(1~{R},2~{S})-2-[[(5-bromanyl-1~{H}-indazol-4-yl)amino]methyl]cyclohexan-1-ol | C14 H18 Br 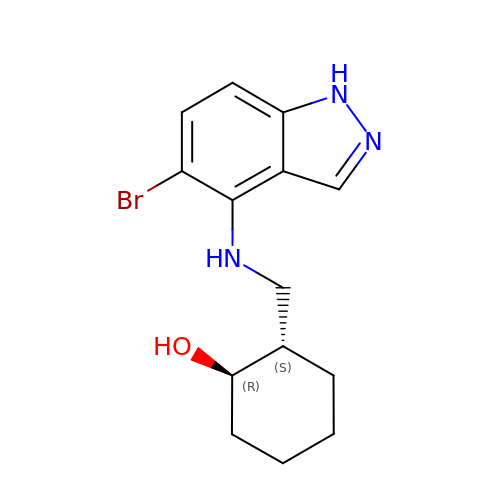N3 O | UQMKMSCULIEFQV-TVQRCGJNSA-N>MEINGVEIEDTFAEAFEAKMARVLITAASHKWAMIAVKEATGFGTSVIMCPAEAGIDCGYVPPEETPDGRPGVTIMI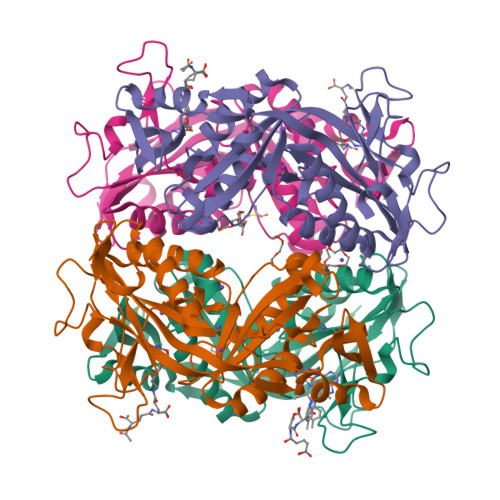GHNDEDELKEQLLDRIGQCVMTAPTASAFDAMPEAEKEDEDRVGYKLSFFGDGYQEEDELDGRKVWKIPVVEGEFIVEDSFGITTGVAGGNFYIMAESQPAGLQAAEAAVDAIKGVEGAYAPFPGGIVASASKVGSKQYDFLPASTNDAYCPTVEDNELPEGVKCVYEIVINGLNEEAVKEAMRVGIEAACQQPGVVKISAGNFGGKLGQYEIHLHDLF[4x]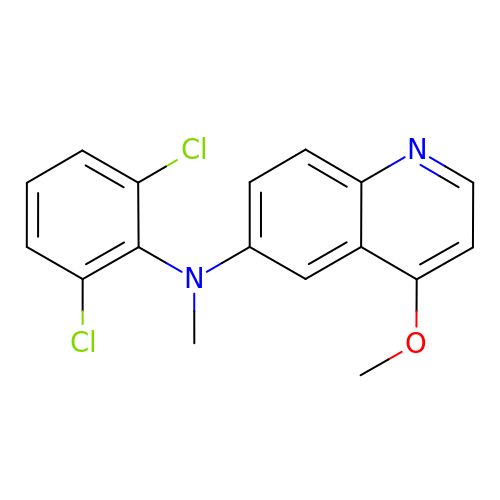N-(2,6-dichlorophenyl)-4-methoxy-N-methylquinolin-6-amine | C17 H14 Cl2 N2 O | IQXIXPLQQDFASE-UHFFFAOYSA-N> DGVFT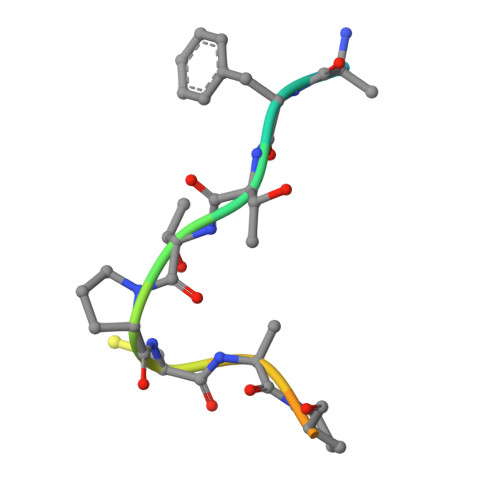TPCDPEYAGG>MPREYEFAEKILFTEEEIRTRIKEVAKRIADDYKGKGLRPYVNPLVLISVLKGSFMFTADLCRALCDFNVPVRMEFICVSSYGEGLTSSGQVRMLLDTRHSIEGHHVLIVEDIVDTALTLNYLYHMYFTRRPASLKTVVLLDKREGRRVPFSADYVVANIPNAFVIGYGLDYDDTYRELRDIVVLRPEVYAEREAARQKKQRAIGSADTDRDAKREFHSKYLEHHHHH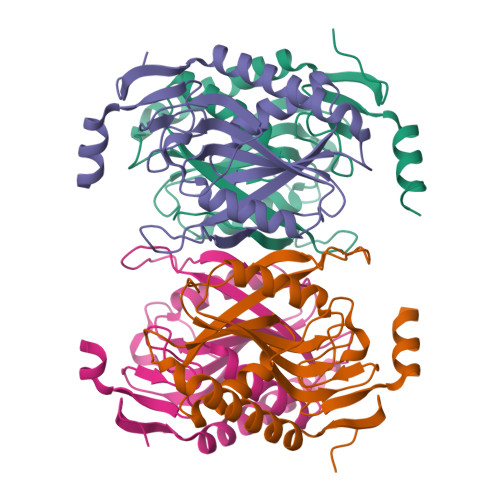H[4x]2-[(2,5-DICHLOROBENZYL)SULFANYL]-5-METHYL[1,2,4]TRIAZOLO[1,5-A]PYRIMIDIN-7-OL 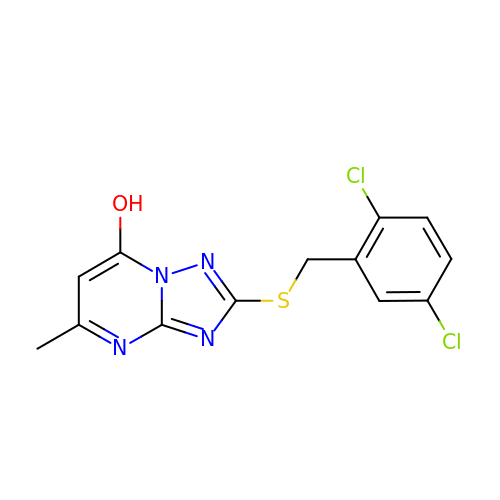| C13 H10 Cl2 N4 O S | VQASKKWJQGYGRL-UHFFFAOYSA-N> MEAPPVTMMPVTGGTINMMEYLLQGSVLDHSLESLIHRLRGLCDNMEPETFLDHEMVFLLKGQQASPFVLRARRSMDRAGAPWHLRYLGQPEMGDKNRHALVRNCVDIATSENLTDFLMEMGFRMDHEFVAKGHLFRK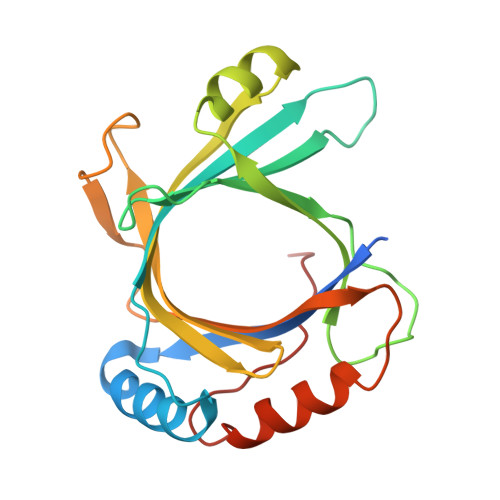GIMKIMVYKIFRILVPGNTDSTEALSLSYLVELSVVAPAGQDMVSDDMKNFAEQLKPLVHLEKIDPKRLM>[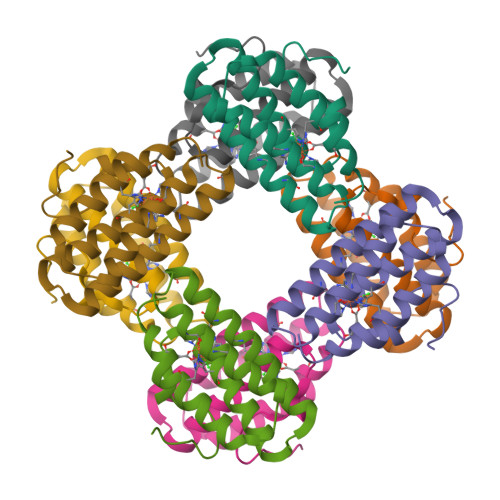8x]MGFPIPDPYVWDPSFRTFYSIIDDEHKTLFNGIFHLAIDDNADNLGELRRCTGKHFLNEQVLMQASQYQFYDEHKKEHETFIHALDNWKGDVKWAKSWLVNHIKTIDFKYKGKI>MGKMEELVKRAEELAKEAKEMLEILKKAHEEGKIDSFLYEALKEMLESIKELAEALKELLEHPTGEKHLEALIKLLKSMVGILASMYEIARYRYLVGQQKQQDPNAPVDPRLPEEAREEAEKYVKEFEELVKKLKDSGKLREVEGLRELLEFLRELAEKTLEAAEEYAKLDPDDELAKGLLEAARRILEALERALRAMEETDEWDLAIAEAAVEIAEAAIELVIKPVVEKLKEGSGHHHHHH[2x]

Here we use a robust deep learning pipeline to design complex folds and soluble analogues of integral membrane proteins. Unique membrane topologies, such as those from G-protein-coupled receptors, are not found in the soluble proteome, and we demonstrate that their structural features can be recapitulated in solution. Biophysical analyses demonstrate the high thermal stability of the designs, and experimental structures show remarkable design accuracy. The soluble analogues were functionalized with native structural motifs, as a proof of concept for bringing membrane protein functions to the soluble proteome, potentially enabling new approaches in drug discovery.

Then, we tested our design approach in one of the most prevalent membrane folds in nature: the GPCR fold. The core topology of GPCRs comprises seven transmembrane helices that facilitate numerous non-local interactions, enabling them to bind to a variety of ligands, including photoreceptors, odours, pheromones, hormones and neurotransmitters. De novo design of GPCR-like folds (GLFs) offers the potential to create new small-molecule receptors and protein scaffolds with functional sites of GPCRs. We tested 56 designs, of which 36 were expressed to be soluble, and we selected the ten most highly expressed designs for further biochemical characterization. Of these ten designs, nine were monodisperse monomers in solution, and all showed the characteristic circular dichroism signature of α-helix-rich proteins. All ten designs also showed high thermal stabilities (Tm > 90 °C). Last, the designed GLFs preserved the canonical seven-helical bundle characteristic of native GPCRs. Structurally, the crystal structures were in very good agreement with the design models, with r.m.s.d.Cα values of 1.05 Å and 0.88 Å for GLF_18 and GLF_32, respectively. This accuracy further extended to the side-chain level, for which comparisons of crystal structures versus design models for GLF_18 and GLF_32 showed 1.54 and 1.40 Å r.m.s.d.fa values, respectively. Comparing the structures of the soluble analogues with that of the reference native GPCR, the overall backbone r.m.s.d.Cα values were 3.08 and 3.51 Å for GLF_18 and GLF_32, respectively.> MAVGSRPGRISQELRAIMNLPEGQLPPWCMKMKDIGLPTGYPDLKIAGLNWD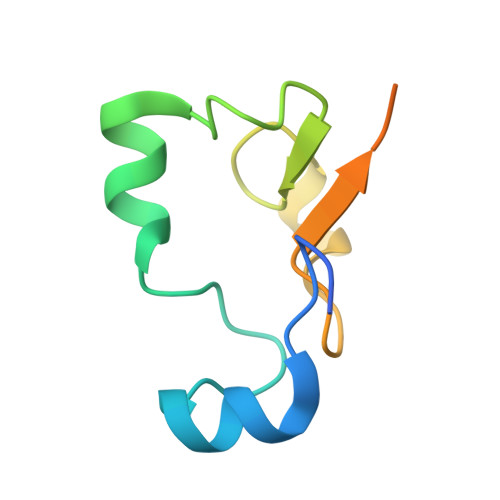ITNLKGDVYGKIIPNHHSRSKKQGRNYFGALI> MAASQTSQTVASHVPFADLCSTLERIQKSKGRAEKIRHFREFLDSWRKFHDALHKNHKDVTDSFYPAMRLILPQLERERMAYGIKETMLAKLYIELLNLPRDGKDALKLLNYRTPTGTHGDAGDFAMIAYFVLKPRCLQKGSLTIQQVNDLLDSIASNNSAKRKDLIKKSLLQLITQSSALEQKWLIRMI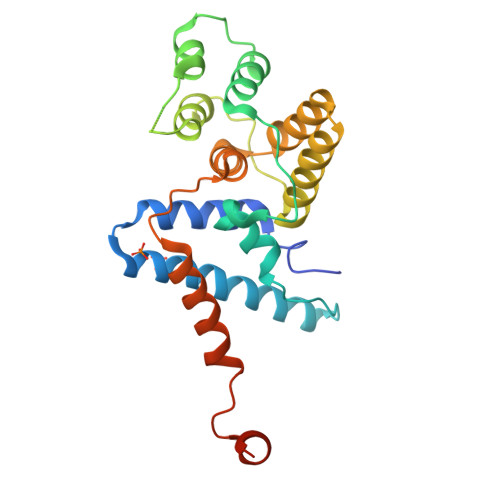IKDLKLGVSQQTIFSVFHNDAAELHNVTTDLEKVCRQLHDPSVGLSDISI8-demethyl-8-aminoriboflavin-5'-phosphate | C16 H19 N5 O9 P | 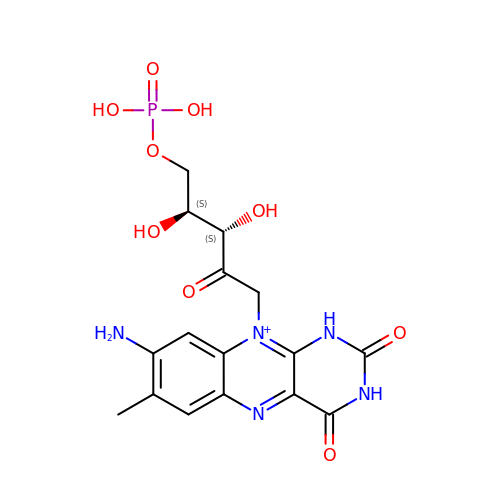SDTLZDHOYFRAPQ-WCQYABFASA-O1,3,3-trimethyl-2-[(1E,3E)-3-methylpenta-1,3-dien-1-yl]cyclohexene | C15 H24 | 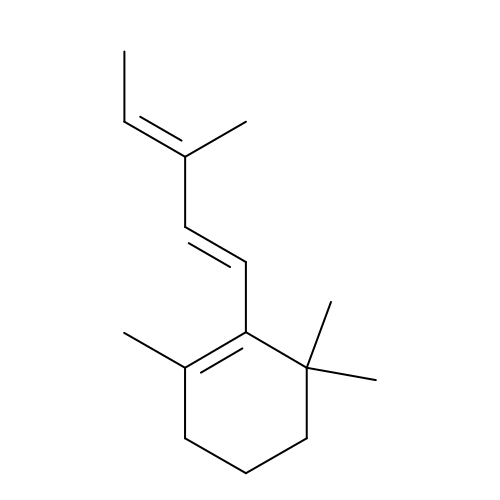KUEVAPFABUUVHS-AYCKBHPDSA-N> PRRPKFLAWGEPVVLSLLLLLCLVLGLALAALGLSVHHWDSPLVQASGGSQFCFGLICLGLFCLSVLLFPGRPSSASCLAQQPMAHLPLTGCLSTLFLQAAETFVESELPLSWANWLCSYLRGLWAWLVVLLATFVEAALCAWYLIAFPPEVVTDWSVLPTEVLEHCHVRSWVSLGLVHITNAMLAFLCFLGTFLVQSQPGRYNRARGLTFAMLAYFITWVSFVPLLANVQVAYQPAVQMGAILVCALGILVT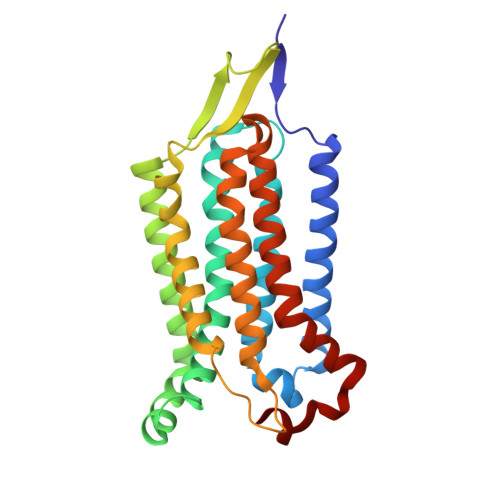FHLPKCYVLLWLPKLNTQEFFL>HMDKLPNIVILATGGTIAGSAATGTQTTGYKAGALGVDTLINAVPEVKKLANVKGEQFSNMASQNMTGDVVLKLSQRVNE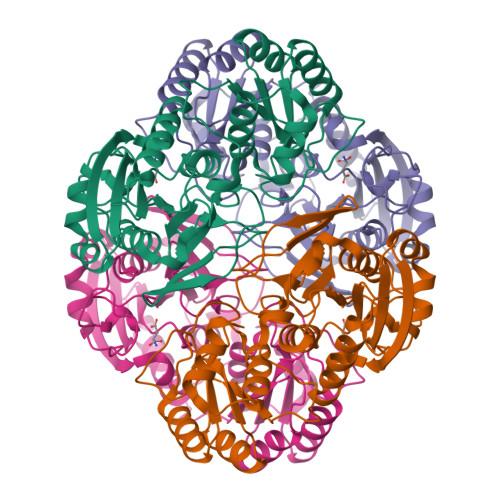LLARDDVDGVVITHGTDTVEESAYFLHLTVKSDKPVVFVAAMRPATAISADGPMNLLEAVRVAGDKQSRGRGVMVVLNDRIGSARYITKTNASTLDTFKANEEGYLGVIIGNRIYYQNRIDKLHTTRSVFDVRGLTSLPKVDILYGYQDDPEYLYDAAIQHGVKGIVYAGMGAGNVSVRGIAGMRKAMEKGVVVIRSTRTGNGIVPPDEELPGLVSDSLNPAHARILLMLALTRTSDPKVIQEYFHTY[3x]> MAKIAYFKGLEQFILENSLIKNKPIKIVIGISMQSPHQISNEHKQSGDSFRAFVDLLRKTNEQCIRDENNNESAIRISELIVVITDGLHRHNLRLYKNVSTTEAESEAAGLGQKWVADNRQFLEAIGQCGISYKVIHWEELKSVAFNRYLQIVEEEYEKPNSEFRSIIDNLTQTHLEKLVNFLLETRDSSFTQEDCVSATRKYLLEEAASAFEFASLKADGMTYPGPCSPGFKYIYDTYLSESNPLPFIEYGMRGGKKLPSFWKEESPVENALSGMPDEEFLIHHTSNFSNHHHHHH

Cyclodipeptide synthases (CDPSs) are enzymes that use sequentially two aminoacyl-tRNAs (aa-tRNAs) to catalyze the formation of two peptide bonds leading to the production of various cyclodipeptides (Gondry et al. 2009; Canu et al. 2019). CDPSs are built around a Rossmann fold similar to the catalytic domain of the two class Ic aminoacyl-tRNA synthetases (aaRSs), TyrRS and TrpRS. Overall, the data show that the first aa-tRNA binds the enzyme with its aminoacyl moiety accommodated in a P1 pocket. Here, we study the binding of E. coli phenylalanyl-tRNAPhe (Phe-tRNAPhe) to the XYP-CDPS from Candidatus Glomeribacter gigasporarum (Cglo-CDPS) by gel filtration and electrophoretic mobility shift assay.

Moreover, we showed that the replacement of the conserved catalytic serine residue S32 by an alanine (Cglo-CDPS-S32A) inactivated the enzyme. Therefore, this variant allows formation of a CDPS:aa-tRNA complex without further reaction. The 5.0 Å resolution structure of the Cglo-CDPS-S32A:Phe-tRNAPhe complex shows a Phe-tRNAPhe molecule bound to a monomer of Cglo-CDPS. To avoid overfitting, the protein was refined as a polyalanine model with only a few side chains modeled for residues visible in the electron density. The structure shows that Cglo-CDPS approaches Phe-tRNAPhe from the major groove of the acceptor stem via the β2 and β7 strands of the first half of the Rossmann fold. The CCA arm is bent and located in a channel delineated by the two catalytic loops CL1 and CL2. This contributes to the positioning of the aminoacyl group in the catalytic pocket of the enzyme. Comparison of the structure of free tRNAPhe with that of Phe-tRNAPhe bound to Cglo-CDPS (rmsd = 3.8 Å for 1611 atoms compared), highlights the bending of the aminoacylated CCA end of Phe-tRNAPhe that accompanies the positioning of the aminoacylated terminal adenosine 76 in the catalytic pocket. In the final steps of the refinement procedure, weak residual density was visible in the active site at the position expected for the phenylalanyl moiety. The binding mode allows positioning of the esterified phenylalanine within the catalytic pocket close to the catalytic serine residue.>GHMSYGVRLHVWGERALFTRPEMKVERVSYDIITPSAARGILEAIHWKPAIRWVVDSIQVLKPICFESIRRNEVGSKLSAASISKAIKAGRTDELVKYVEEDRQQRAATVLREVGYIIAAHFEMTDKAGPDDNVGKHLDIFNRRARRGQCFQAPCLGTREFPA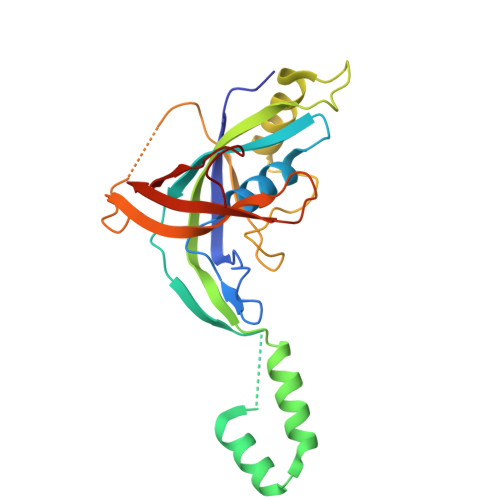SFALLGDDDTPPASDPALSGERDLGWMLHDIDFADGMTPRFFRARMVDGLVAVPPPQDGGVRA[2x]>GGTTGGTGTGGTTGG[2x]

Here, we report three Pb2+-complexed structures of the thrombin binding aptamer (TBA). These high-resolution crystal structures showed that TBA forms intramolecular G-quadruplex and Pb2+ is bound by the two G-tetrads in the center. Each TBA molecule folds into an antiparallel chair-like quadruplex, which can be divided into four regions: two TT linkers (T3T4 and T12T13), one TGT linker (T7G8T9) and the central G-tetrads. The Pb2+ ion resides in-between the two G-tetrads, coordinating with the eight O6 atoms of the G-tetrads.

The A-form structure belongs to the tetragonal space group P41212; it contains two TBA-Pb2+ complexes per asymmetric unit. Compared to the B-form structure, the resolution (1.4 Å) of the A-form TBA-Pb2+ complex structure is higher, therefore it was used for further structural analysis. The two TBA-Pb2+ complexes assembled into one dimer in the A-form structure. For the AB (or CD) dimers in the A- and B-form structures, T3 and T4 arrange in two layers; similar conformations were also adopted by T12 and T13. However, instead of T12 or T13 from the same molecule, T3 and T4 form hydrogen (H) bond interactions with T13 and T12 from the partner molecule, respectively. In the A-form TBA-Pb2+ complex structure, each TBA molecule captures one Pb2+ ion. The shortest coordination (2.56 Å) forms between Pb2+ and the G1 nucleotide of TBA molecule B. In addition, Pb2+ forms several short coordination (~ 2.60 Å) with other G nucleotides. The average Pb2+–O6 coordinating distance is only 2.65 Å in the A-form TBA-Pb2+ complex structure. The average in-plane N1–O6 and N2–N7 distances are 2.83 Å and 2.85 Å, respectively. Compared to other G-quadruplex structures, both the N1-O6 and N2-N7 distances are shorter in the TBA-Pb2+ complex structure. The two G-tetrads of TBA-Pb2+ complex form stable hydrophobic stacking interactions, the average between-plane O6–O6 distance is only 2.98 Å, which is significantly shorter than other quadruplexes.> SNASDKGKLSLQDVAELIRARACQRVVVMVGAGISTPSGIPDFRSPGSGLYSNLQQYDLPYPEAIFELPFFFHNPKPFFTLAKELYPGNYKPNVTHYFLRLLHDKGLLLRLYTQNIDGLERVSGIPASKLVEAHGTFASATCTVCQRPFPGEDIRADVMADRVPRCPVCTGVVKPDIVFFGEPLPQRFLLHVVDFPMADLLLILGTSLEVEPFASLTEAVRSSVPRL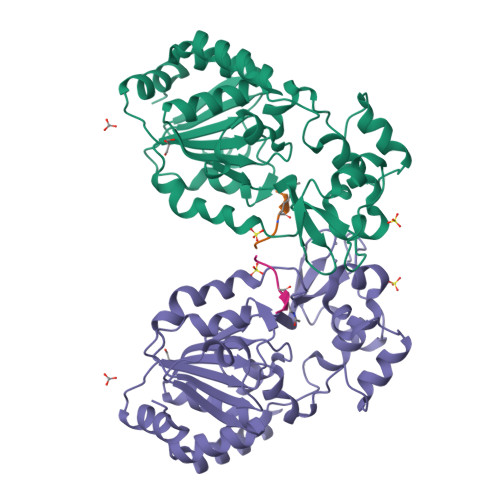LINRDLVGPLAWHPRSRDVAQLGDVVHGVESLVELLGWTEEMRDLVQRETGKLDGPDK;> TRSGKVMRRLLR>[4x]NITVRFVTENDKEGWQRLWKSYQDFYEVSFPDDLDDFNFGRFLDPNIKMWAAVAVESSSEKIIG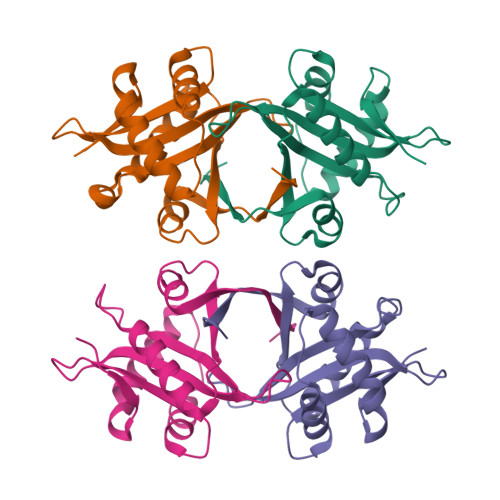MINFFNHMTTWDFKDKIYINDLYVDENSRVKGAGGKLIQFVYDEADKLGTPSVYWCTDESNHRAQLLYVKVGYKAPKILYKRKGY> GKRVLIVDD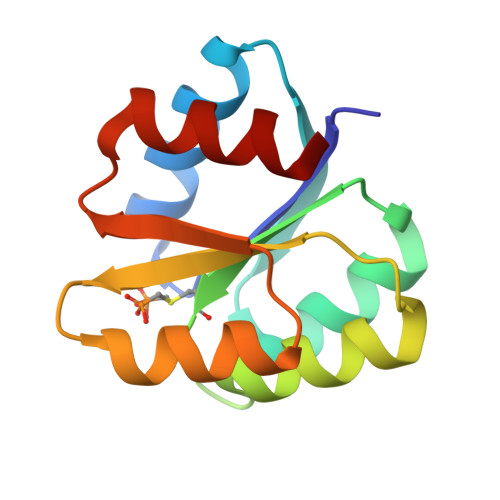AAFMRMMLKDIITKAGYEVAGEATNGREAVEKYKELKPDIVTMCITMPEMNGIDAIKEIMKIDPNAKIIVASAMGQQAMVIEAIKAGAKDFIVKPFQPSRVVEALNKVSK>MSMMAERDMGRILLDLSDDVIQRLDDLKVQRNIPRAELLREAVEQYLEKQDRAKDTISSALGLWQDCEEDGMEYQRQLRKEW[2x];>MTSGSALFDTNILIDLFSGRREAKQALEAWPPQNAISLITWMEVMVG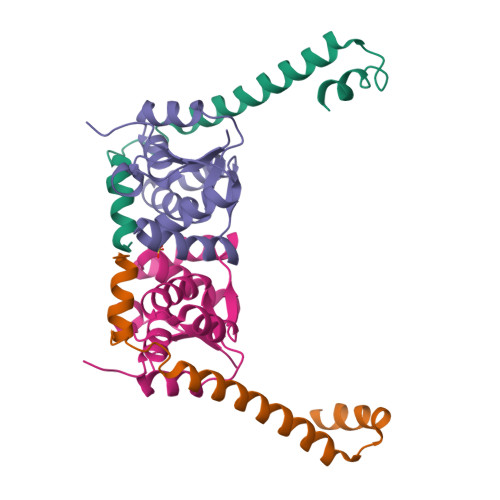AKKYHQEQRTRMALSTFNIINISQDIAERSVALRQEYKLKLPDAIILATAQLHRLELITRNTKDFAGIPGVVTPYEIHPE[2x]>[2x]MRGSHHHHHHGSVTCTGCVDLDELSFEKTVERFPYSVVKFDIAYPYGEKHEAFTAFSKSAHKATKDLLIATVGVKDYGELENKALGDRY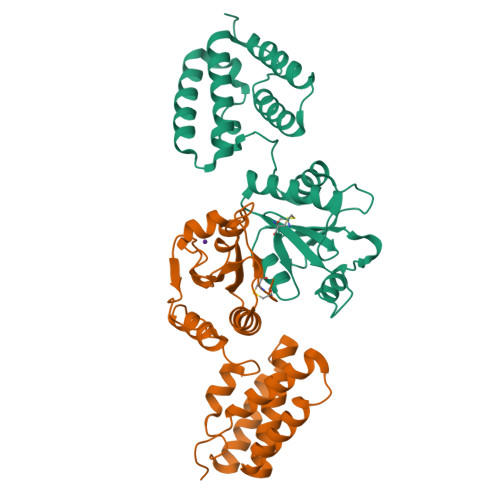KVDDKNFPSIFLFKGNADEYVQLPSHVDVTLDNLKAFVSANTPLYIGRDGCIKEFNEVLKNYANIPDAEQLKLIEKLQAKQEQLTDPEQQQNARAYLIYMRKIHEVGYDFLEEETKRLLRLKAGKVTEAKKEELLRKLNILEVFRVHKVTKTAPEKEEL> DNSIFGDTKSESKQLGNTSSVANTPSEIPDAHKAEQEDIIEKTESVDKKVDSGEERNEQEREIMNDHSKSANPKKTTITRVEPETFEIPQAHEIV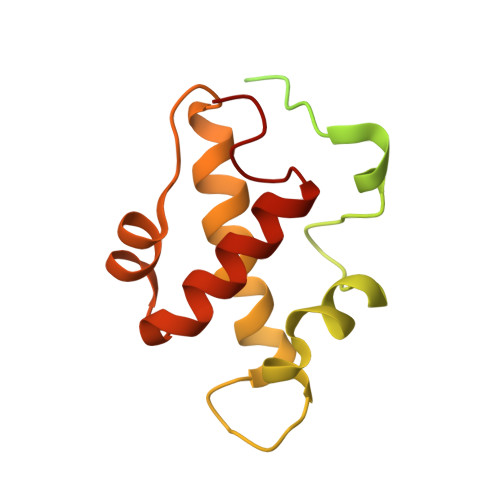IPSYSKWFNLEKIHSIEVQSLPEFFTNRIPSKTPEVYMRYRNFMVNSYRLNPNEYFSVTTARRNVSGDAAALFRLHKFLTKWGLINYQVDSK>[6x]GMPTLPKAEAKELSAFVQSCVEYKTNVCFTDVAAYESNQKGVLSSGLAVLVGTHKQLRDPAVQRLPFYNPAVAEAIERVKEGGTYGVLVEGLANAAGSKFVRVVVGEVPTKASRNNCPARPDVVTALVTAALDEVKEPNTTVDVFVLSNAVLPIAAAVARCGKHNFSAKD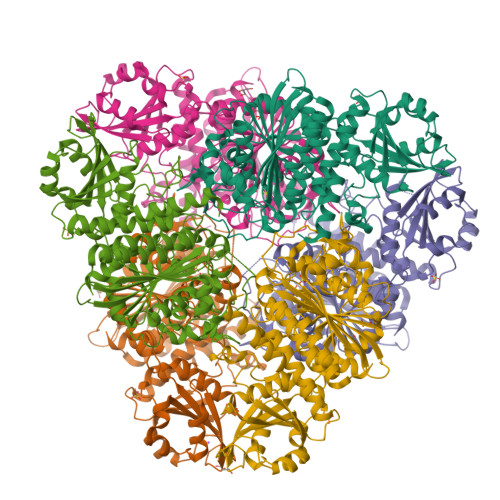GAAAAAYNSGKVSRLQVVFPEPPAIPPKDLEAVATSTQLCQRLVDAPPNLLTTATFTEIAQGYAKALGFDVDVICGDDLCERGYGGIYSVGKAAFEAPRLVTLLYTPKGTPVKKVSLVGKGIVYDCGGLALKPADYMKLMKHDMGGAAAVFCGFLTAVRLQQPVQLSCTLCLAENAIGPKSYRNDDIIVMKSGKTVEVINTDAEGRIVLGDGVFHATNELSFTPDVVIDMATLTGAQGIATGRHHAGLYVNEEGAEAAMLRAGRESGETCFPVLYCPEYHEPEFKSNHADMTNLMERRDNAGVSCAGYFITTHLSPKFTGAHIHVDLAYPVFNSNGATGFGPALLTEYFRKL>[8x]GDTKEQRILRYVQQNAKP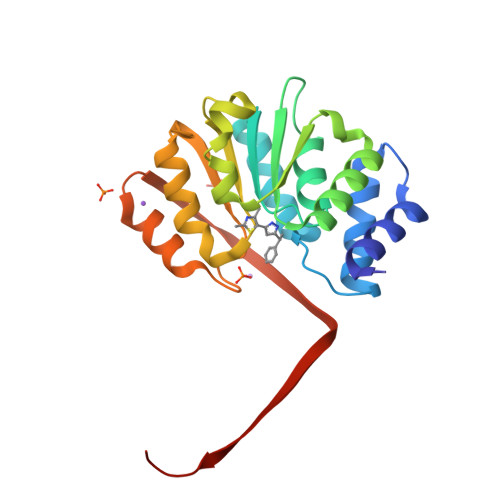GDPQSVLEAIDTYCTQKEWAMNVGDAKGQIMDAVIREYSPSLVLELGAYCGYSAVRMARLLQPGARLLTMEINPDCAAITQQMLNFAGLQDKVTILNGASQDLIPQLKKKYDVDTLDMVFLDHWKDRYLPDTLLLEECGLLRKGTVLLADNVIVPGTPDFLAYVRGSSSFECTHYSSYLEYMKVVDGLEKAIYQGPSSPS>[2x]MRGSHHHHHHGSMAEKNYVMAIDQGTTSSRAIIFDRNGKKIGSSQKEFPQ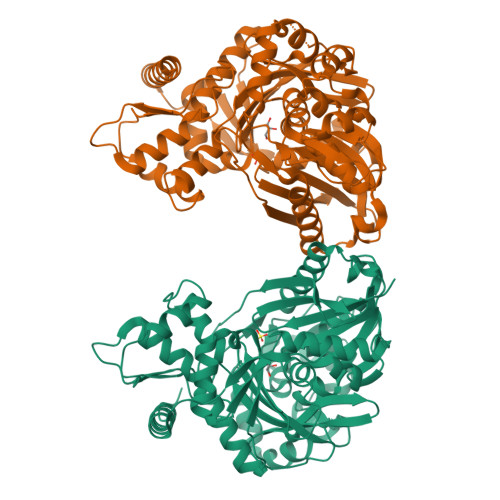YFPKSGWVEHNANEIWNSVQSVIAGAFIESGIRPEAIAGIGITNQRETTVVWDKTTGQPIANAIVWQSRQSSPIADQLKVDGHTEMIHEKTGLVIDAYFSATKVRWLLDNIEGAQEKADNGELLFGTIDSWLVWKLTDGQVHVTDYSNASRTMLYNIHKLEWDQEILDLLNIPSSMLPEVKSNSEVYGHTRSYRFYGSEVPIAGMAGDQQAALFGQMAFEKGMIKNTYGTGAFIVMNTGEEPQLSDNDLLTTIGYGINGKVYYALEGSIFVAGSAIQWLRDGLRMIETSPQSEELAAKAKGDNEVYVVPAFTGLGAPYWDSEARGAVFGLTRGTTKEDFVRATLQAVAYQSKDVIDTMKKDSGIDIPLLKVDGGAAKNDLLMQFQADILDIDVQRAANLETTALGAAYLAGLAVGFWKDLDELKSMAEEGQMFTPEMPAEERDNLYEGWKQAVAATQTFKFKAKKEGE> MNKRHALLLTAVLGMATAYAQTAPTTTTVNTLQTVYRDPSLTSAPITANVGKYVGPLSTFLASIAKSAGYEVVFNFNIDALALINGEIVFGNSTASVTTSYATPLGRPQELPAKPVVHNFSNAPFNEAWPLLMDVYELDYQLVKVGSANVIRIGQRPKQLALPLKFISAESALTAIEKFFGEEKFETVISLDSNN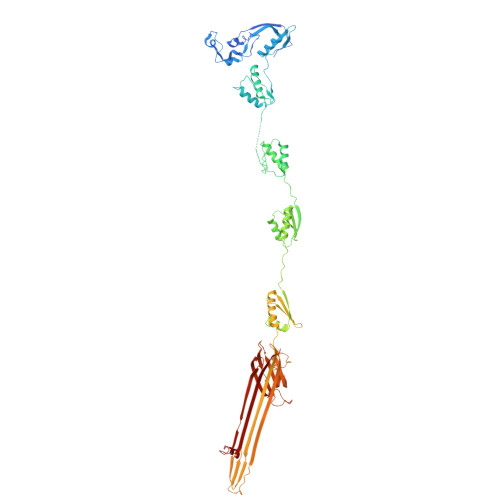KPFQTTRPTGKFGLPNSIKVIPDSSNKRLIIGSNSEDGIRIRSFVETIDVQSSGKVISTDSISEIYIVRGQKESVLQFLRDSFPELIVTDYASGGLAIEGPRTSVNRAIILLGQVDRAPEIPIVQRIYTVRGQAADITALLAAQYPTLRVTPVGQTGQLVLNGAQAQLDTALALLEQVDRPAPVAESRTVQRVFQLVNASAEEVKATLEGTLARDLTADSNNDVLPNVPVTATDANGNTTVVSVPNALGKTANQGTANAQAQTAQTPANTQQATLIADKRTNSLIVRGTPEQVAQVAELVPQLDQVVPQINVQVRIQEVNERALQSLGLNWRATFGGFNVAVSGGTGLAATFNPTQSFLGFNIFPTLTALETQGLTRRVYDGNVTMQSGQRSLSATGGAQNASSGAAASVKSGGRLEINIPSAAGNIVRQIDYGLNLDFFSPQVAPDGTITLRIRGQVNQPATAITADSLPNLIDFTNSEAQSTITFKNGQTILMSGLLGSTETTNRSGVPFLSSLPGVGAAFGEKRTEKTQSQLLVIITGTVVK>MAIETNAVVITDLNPLYPRDRDYIYEGAAQIRLIKQTLQNTFPNVTEPVDIDSDTFKIMSEKLKFTGDAMDVGGLMIKNVTPGTGDKDVVTKGQMEAFMKNWMENKLYRIGSYYITEEDINPGDSISLGFGSWAKVTGVIMGTGVVNPDGSVPNAQRVEFQAGGTGGRVFNTIRTENVPLMTVNGSSFSLSSNTHSHNMVFGRGDASGHNSSPNWYSPGGGYSQRTDNDTHTHTISGSVSLGRDDISRQPINTLPPFRAAHIWRRIS[3x];>MIVYNNQAPDAVNNVGQFGATEGSIGAYKQAAEYAADSKYWALLAESKFGTIDDLIAEVERLYQQGVLMKQDIEDLKQDFKDQDARLMSLIAQTNAAVSDANNAVALINQKLIEVQNQLDVLLGMSVDVTTLPPGTPATGSFNPNTGVISLGIPEGEPGKDGSVKDLDTAPTGVPELGDLGFYVDKDDNTVHKTTLENIANLTPSVRSVSVNGGPALDGEVALTINKETVGLGNVLNVAQYSRQEINDKFDKTTKTYQSKAEAYADAQYRQVGEKVLVWEATKYEFYTVAANKTLTPVKTEGRILTVNSRSPDSSGNIDITIPTGNPSLYLGEMVMFPYDPSKNISYPGVLPADGRLVSKESASDLGPSLVSGQLPVVSETEWQSGAKQYFSWGKLADGITDADSTNFINIRLPDWTGGEAIRAPDSDKDSQYNGSVQAQKPYVVTVNNQAPDEITGNVNISRSILGAASSGANSDITSLSGLTTPLSISQGGTGAKDAASARSNLGLGSVSTLDNVPIASGGTGAGDAAGARFNLGLGNSATMNTGTNSDNVLKVGDFGIGRPDGALVFDTTSQDQLLAGLDTYGLCVFRNNQQIAAPWDIWNYSSNLFFRAGDTYSMISIPFESAGKIKVFGGASGSGWKTSRTVYDTVNTTVDVNGFIKAASPIVKVFHDGSFETNEQSDGVSVKKISTGVYLISGCLGLNSDAGWGGVDGGFEIPIDRNKQPRVWLDYEVKEDGSLLIKTYHRTHSTSPAFARNELEGFSDGDPVDIPKDAFISVRVEMPSK[3x];> MALYPIKSLGAVGVIADQAPTDLAPNAFTNAINARFVEQRVFKTGGNAPLSYVDEDKDLTPLSFVSMPFDYYSAGNSFLVVGTNKKLYKLTDESLTDISRKVATVTKKASASIKIYPVVSQIVPKESTISMNFNQTKNLEVSLLPADANNTNLIWEVSNSSYGSITVDPSDSKLATLTSFEKEGNLVVTISTANESVVAQIAVNIIDGDSGIFLSQDTVTIRKGGTTTLTAVTGKTPVTWSSNNASIVSVTPNANSLTAVITANGEGNVTITADNGTKTASCEIVSIPQIDSISLSQSDVTVSRGSQYILTATLSPANAPNQNITWTSSNPNIATVSGTSTQGTINALLAGFTEITATTEEGNRVAVCTVRVDLAGRTMRTSAMAFAAPVSESVETQEEEVVTPPESEETVYFAEPTSGIDTSGMYEGNNFYDYSNVNDIEGFARASLLATPLSSVTLDIVSASLDVGEEIVITATASPEGEYSYQWSVDKTGYVSTTSVTGKSIKLVALRKGEINVTCTVSQMTQKDYDAFDDYPWYHAVISNCAVATTHYETPQVKEFESEYFVDLPGWGEQTVVDNDGNPSVKKFNWKCERVRSFNNRLFALNMREANASGVTTNYPLRLRWSNFANENKAPTLWDDFAYDRVVSSDLASNIVGQTQALENGYAGYIDLADSNGSLIDILPLKDYLFVYTEFETYIGSPTNNTYQPLMFKKLFNDSGILAPECVVEVEGSHFVVTQNDVILHNGATKKSIASNRVKNMLINEVCLVNPLATRVHLHQDKKEVWVLYVGPGEPKESFACTKAAVWNYEFDTWSFRTIPYAQCIGLVDPPVLERGPIWSDFQEITWDDPSIKELVWRKDATNFRQRVTIVGSFLKGFYQVDVGALDYFYDRLNDVVIEKPLEMRLERTGIDFDNVTNEWNQKHINRFRPQTTGSGTYIFEAGGSQFSNEYGHPHTSKTYTIGVDRHVSVRLNHPYLFYNVIDNDVNSNAAINGLTIEFAVGGRR;>MAMPDVQYPINTYGWLKKAVALWADRDDDEFVNQIPNFINFAEKEIYRNLRIPPLEKEVYLDIKDGVAYIPPDYLEAQWMMRAKDGTIFQVTSPEEISYRRQHGTINPSHWNNQPVNFARFGSRFIFYPSIEADTPYYPDDGSPLIPAENSVILSYYADPPEFHEDTDTSTILTIAPELLLYFTLRHACLFVQDDNGVQKWSALGKAILDEMVEQNKKQEYSGSPIAIPNNMTRLQSSLPDIYGIRTSRV[2x];>[2x]MAKQKYSEEVLDELRVDLQRRFNYAQGYVDMAVKGYAREAWEYFYGNLPAPVTAGSSSWVDRTVWESVNGTLQDIINVFCSGDEAVTFVADNQQDSDAADVATKLVNQILLRDNPGYNIISSAAQECLVTRNSFIKYYWDEQTSTQTEEAEGVPPEALAAYVQGLEAGGLKNLEVFTEENEDGTVDVKVTYEQTVKRVKVEYVPSEQIFVDEHATSFADAQYFCHRVRRSKEDLVAMGFPKDEIEAFNDWTDTMDTTQSTVAWSRTDWRQDIDADIGTDTEDIASMVWVYEHYIRTGVLDKNKESKLYQVIQAGEHILHTEEVTHIPFVTFCPYPIPGSFYGQSVYDITKDIQDLRTALVRGYIDNVNNANYGRYKALVGAYDRRSLLDNRPGGVVEMERQDAIDLFPYHNLPQGIDGLLGMSEELKETRTGVTKLGMGINPDVFKNDNAYATVGLMMNAAQNRLRMVCRNIAHNGMVELMRGIYNLIRENGEVPIEVQTPRGMIQVNPKQLPARHNLQVVVAISPNEKAERAQKLISLKQLIAADAQLAPLFGLEQDRYMTAQIFELMGIKDTHKYLLPLEQYQPPEPSPMEILQLEMTKAQVENVQASSQKMIADAFDQRERTTFEQQKAADELSLRQEELQFKQENAADAMTLENRKEDNNATLEQAKHKLALMQQQVRQYESVLKELQMVMSHQVDQEKIVQQARVQDKTLELQKKEANVTKKEQQASLKDSRIPGKRLGSKK

Escherichia coli phage SU10 belongs to the genus Kuravirus from the class Caudoviricetes of phages with short non-contractile tails. Here we show that the virion of SU10 has a prolate head, containing genome and ejection proteins, and a tail, which is formed of portal, adaptor, nozzle, and tail needle proteins and decorated with long and short fibers. In contrast to other short-tailed phages, the tails of Kuraviruses elongate upon cell attachment. After binding to the host, SU10 tail, nozzle proteins, and short fibers re-arrange to form a nozzle that extends the tail.

The genome release intermediate of SU10 b, d lacks the tail needle and contains a 277 Å-long nozzle formed by short tail fibers and nozzle proteins. The tail of the SU10 genome release intermediate is reorganized into the nozzle built from nozzle proteins and short tail fibers. To form the nozzle, the four nozzle domains undergo an extensive structural change from the L shape in the SU10 virion to the straight arrangement in the genome release intermediate. In the new conformation, the four domains form a line pointing away from the portal complex. While the interaction of the short tail fiber dock loop with a short tail fiber remains preserved, the connections of the short tail fiber loop to the beta-propeller domain rotate about each other and bend 135° to point away from the phage head. The same rotation is performed by the short tail fiber. In the new arrangement, the nozzle proteins and short tail fibers alternate to form a nozzle that prolongs the tail by 277 Å. Furthermore, the distal part of the beta-propeller domain of the nozzle protein shifts 3 Å away from the tail axis, resulting in a broadening of the tail channel. The structures of the SU10 virion and genome release intermediate differ in the direction in which the long tail fibers point away from the adaptor complexes. The long tail fibers in the genome release intermediate are rotated 6.6° relative to their orientation in the virion.> MRLLSSLSGSSVSSDAEEYQPPIWKSYLYQLQQEAPRPKRIICPREVENRPKYYGREFHGIISREQADELLGGVEGAYILRESQRQPGCYTLALRFGNQTLNYRLFHDGKHFVGEKRFESIHDLVTDGLITLYIETKAAEYISKMTTNPIYEHIGYATLLREKVSRRLSRSKNEPRKTNVTHEEHTAVEKISSLVRRAALTHNDNHFNYEKTHNFKVHTFRGPHWCEYCANFMWGLIAQGVRCSDCGLNVHKQCSKHVPNDCQPDLKRIKKVYCCDLTTLVKAHNTQRPMVVDICIREIEARGLKSEGLYRVSGFTEHIEDVKMAFDRDGEKADISANVYPDINIITGALKLYFRDLPIPVITYDT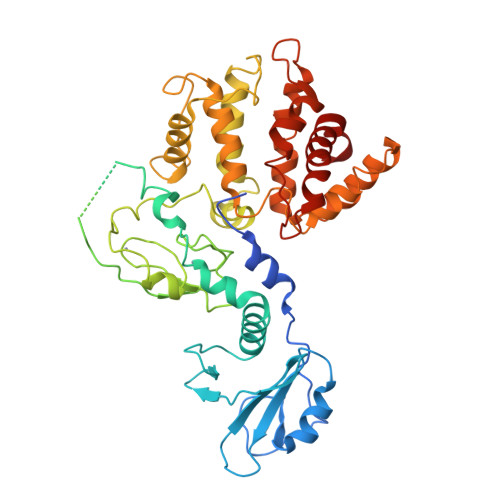YSKFIDAAKISNADERLEAVHEVLMLLPPAHYETLRYLMIHLKKVTMNEKDNFMNAENLGIVFGPTLMRPPEDSTLTTLHDMRYQKLIVQILIENEDVLF> MWDS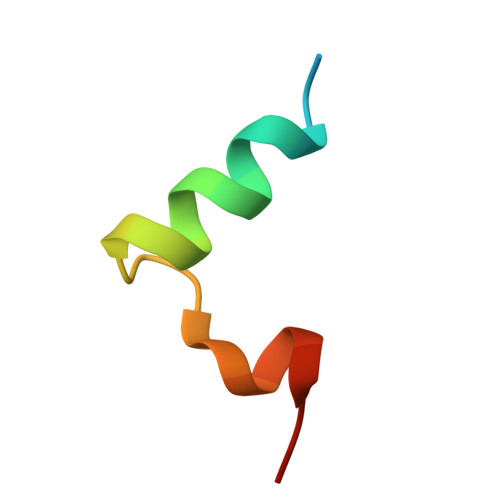SYMQQVSEGLMTGKVPIDQVFGAN Monensin A is a prototypical natural polyether polyketide antibiotic. Biosynthesis of monensin A involves construction of a polyene polyketide backbone, subsequent epoxidation of the alkenes, and, lastly, formation of cyclic ethers via epoxide-opening cyclization. MonCI, a flavin-dependent monooxygenase, is thought to transform all three alkenes in the intermediate polyketide premonensin A into epoxides. MonCI is a class A flavin-dependent monooxygenase based on its structural and biochemical features.

To elucidate the structural basis of MonCI’s catalytic activity, we determined the MonCI crystal structure at 1.9 Å resolution using the multi-wavelength anomalous diffraction method. Two molecules of MonCI are present in the crystal asymmetric unit (chain A and B). One FAD coenzyme and one chloride ion were found in each chain. MonCI consists of a β-strand-rich substrate-binding domain located near the C-terminus and a Rossmann-like three-layer ββα sandwich FAD-binding domain located near the N-terminus. The FAD- and substrate-binding pockets are fused and form a continuous chamber that is shaped like an inverted letter L. The substrate-binding pocket, which lies immediately on top of the isoalloxazine ring of FAD, is about 40 Å long and about 25 Å wide. The volume of the fused FAD- and substrate-binding pocket of MonCI is 995 Å3, as calculated using the program CASTp 3.036. FAD is bound noncovalently to MonCI through numerous direct and solvent-mediated interactions. The chloride ion coordinates with five hydrogen bond donors (Gln52 main chain nitrogen, Ser298 side chain hydroxyl group, and three water molecules) in a distorted trigonal bipyramidal stereochemistry. In our MonCI crystal structure, the FAD is in the “in” conformation, which is the expected conformation during epoxidation.

>[2x]MNHKVHHHHHHIEGRHMTTTRPAHAVVLGASMAGTLAAHVLARHVDAVTVVERDALPEEPQHRKGVPQARHAHLLWSNGARLIEEMLPGTTDRLLAAGARRLGFPEDLVTLTGQGWQHRFPATQFALVASRPLLDLTVRQQALGADNITVRQRTEAVELTGSGGGSGGRVTGVVVRDLDSGRQEQLEADLVIDATGRGSRLKQWLAALGVPALEEDVVDAGVAYATRLFKAPPGATTHFPAVNIAADDRVREPGRFGVVYPIEGGRWLATLSCTRGAQLPTHEDEFIPFAENLNHPILADLLRDAEPLTPVFGSRSGANRRLYPERLEQWPDGLLVIGDSLTAFNPIYGHGMSSAARCATTIDREFERSVQEGTGSARAGTRALQKAIGAAVDDPWILAATKDIDYVNCRVSATDPRLIGVDTEQRLRFAEAITAASIRSPKASEIVTDVMSLNAPQAELGSNRFLMAMRADERLPELTAPPFLPEELAVVGLDAATISPTPTPTPTAAVRS> MMGNNMRKLFSMIANSKDKKEKLIESLQ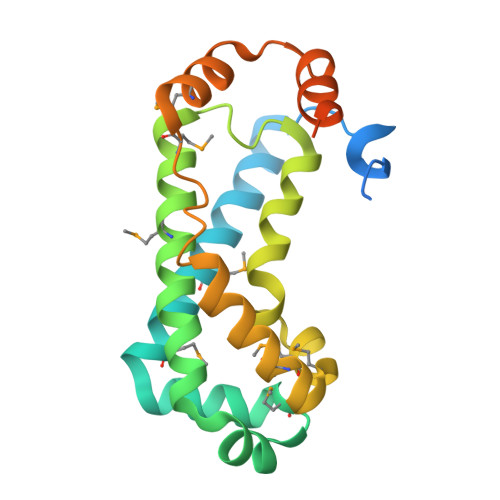ENELLNTDEKKKIIDQIKTMHDFFKQMHTNKGALDKVLRNYMKDYRAVIKSIGVDKFKKVYRLLESETMELLHAIAENPNFLFSKFDRSILGIFLPFFSKPIMFKMSIREMDSQIELYGTKLPLLKLFVMTDEEMNFYANLKTIEQYNDYVRDLLMKFDLEKYMEEKGVQNALEHHHHHH>UGCGUCACACCGGUG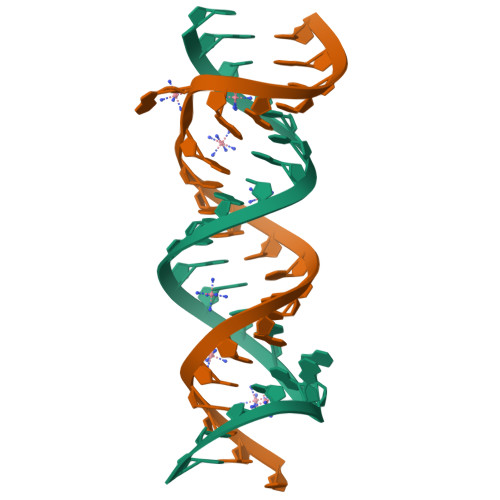AAGUCGC[2x]>VDMSNVVKTYDLQDG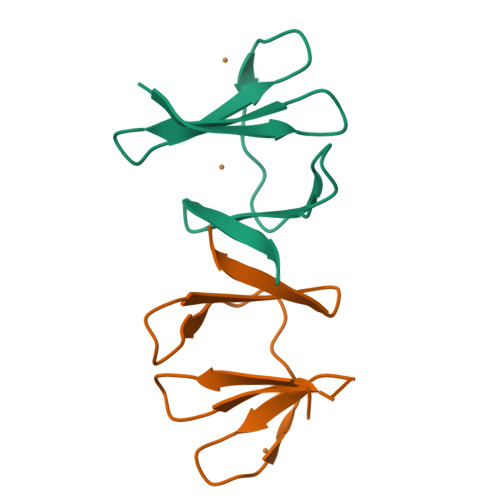SKVHVFKDGKMGMENKFGKSMNMPEGKVMETRDGTKIIMKGNEIFRLDEALRKGHSEGG[2x]> MEKTTEGAFYTREYRNLFKEFGYSEAEIQERVKDTWEQLFGDNPETKIYYEVGDDLGYLLDTGNLDVRTEGMSYGMMMAVQMDRKDIFDRIWNWTMKNMYMTEGVHAGYFAWSCQPDGTKNSWGPAPDGEEYFALALFFASHRWGDGDEQPFNYSEQARKLLHTCVHNGEGGPGHPMWNRDNKLIKFIPEVEFSDPSYHLPHFYELFSLWANEEDRVFWKEAAEASREYLK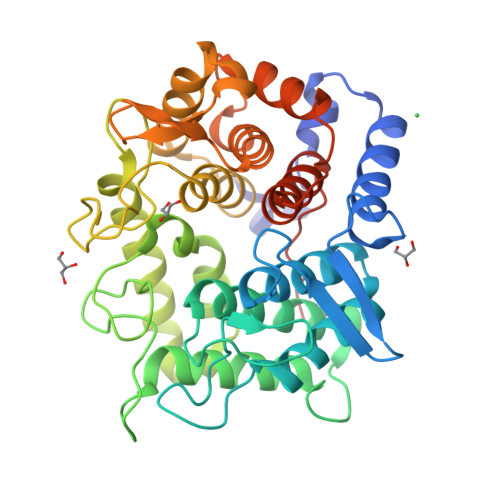IACHPETGLAPEYAYYDGTPNDEKGYGHFFSNSYRVAANIGLDAEWFGGSEWSAEEINKIQAFFADKEPEDYRRYKIDGEPFEEKSLHPVGLIATNAMGSLASVDGPYAKANVDLFWNTPVRTGNRRYYDNCLYLFAMLALSGNFKIWFPEGQEEEHLEHHHHHH>[12x]MATAPRPLREQYLHFQPISTRWHDNDIYGHVNNVTYYAFFDTAVN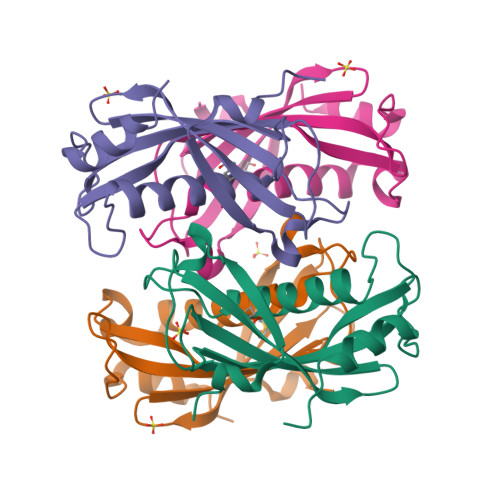TYLIERGGLDIQGGEVIGLVVSSSCDYFAPVAFPQRIEMGLRVARLGNSSVQYELALFLEGQREACAAGRFVHVFVERRSSRPVAIPQELRDALAALQSSAQ> MDWLPRNTNCGGILKEESGVIATYYGPKTNCVWTIQMPPEYHVRVSIQYLQLNCNKES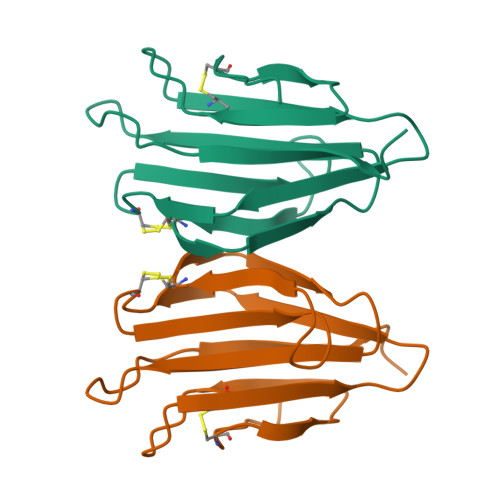LEIIDGLPGSPVLGKICEGSLMDYRSSGSIMTVKYIREPEHPASFYEVLYFQDPQA(2Z,6Z)-3,7,11-trimethyldodeca-2,6,10-trien-1-ol | C15 H26 O 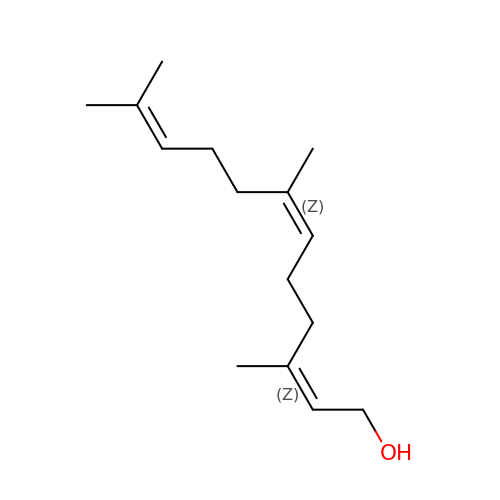| CRDAMVZIKSXKFV-FBXUGWQNSA-N> GLVPRGSHMMEILRGSPALSAFRINKLLARFQAANLQVHNIYAEYVHFADLNAPLNDSEQAQLTRLLQYGPALSSHTPAGKLLLVTPRPGTISPWSSKATDIAHNCGLQQVDRLERGVAYYIEASTLTAEQWRQVAAELHDRMMETVFSSLTDAEKLFIHHQPAPVSSVDLLGEGRQALIDANLRLGLALAEDE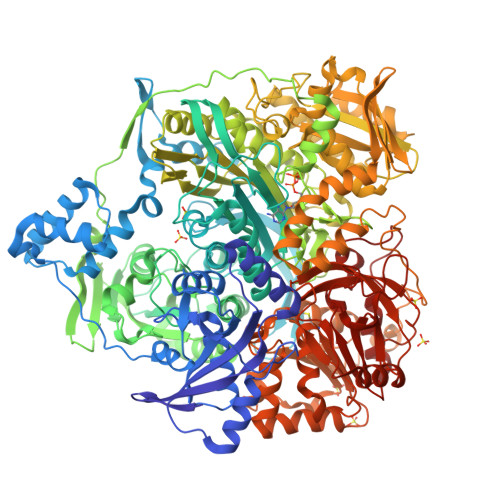IDYLQEAFTKLGRNPNDIELYMFAQANSEHCRHKIFNADWIIDGKPQPKSLFKMIKNTFETTPDYVLSAYKDNAAVMEGSAVGRYFADHNTGRYDFHQEPAHILMKVETHNHPTAISPWPGAATGSGGEIRDEGATGRGAKPKAGLIGFSVSNLRIPGFEQPWEEDFGKPERIVTALDIMTEGPLGGAAFNNEFGRPALTGYFRTYEEKVNSHNGEELRGYHKPIMLAGGIGNIRADHVQKGEIVVGAKLIVLGGPAMNIGLGGGAASSMASGQSDADLDFASVQRDNPEMERRCQEVIDRCWQLGDANPILFIHDVGAGGLSNAMPELVSDGGRGGKFELRDILSDEPGMSPLEIWCNESQERYVLAVAADQLPLFDELCKRERAPYAVIGDATEEQHLSLHDNHFDNQPIDLPLDVLLGKTPKMTRDVQTLKAKGDALNRADITIADAVKRVLHLPTVAEKTFLVTIGDRTVTGMVARDQMVGPWQVPVADCAVTTASLDSYYGEAMSIGERAPVALLDFAASARLAVGEALTNIAATQIGDIKRIKLSANWMAAAGHPGEDAGLYDAVKAVGEELCPQLGLTIPVGKDSMSMKTRWQEGNEQREMTSPLSLVISAFARVEDVRHTLTPQLSTEDNALLLIDLGKGHNALGATALAQVYRQLGDKPADVRDVAQLKGFYDAMQALVAARKLLAWHDRSDGGLLVTLAEMAFAGHCGVQVDIAALGDDHLAALFNEELGGVIQVRAEDRDAVEALLAQYGLADCVHYLGQALAGDRFVITANDQTVFSESRTTLRVWWAETTWQMQRLRDNPQCADQEHEAKANDTDPGLNVKLSFDINEDIAAPYIATGARPKVAVLREQGVNSHVEMAAAFHRAGFDAIDVHMSDLLGGRIGLGNFHALVACGGFSYGDVLGAGEGWAKSILFNHRVRDEFETFFHRPQTLALGVCNGCQMMSNLRELIPGSELWPRFVRNHSDRFEARFSLVEVTQSPSLLLQGMVGSQMPIAVSHGEGRVEVRDDAHLAALESKGLVALRYVDNFGKVTETYPANPNGSPNGITAVTTENGRVTIMMPHPERVFRTVANSWHPENWGEDSPWMRIFRNARKQLG> SDLPMPMRFRHLKKTSKEAVGVYRSPIHGRGLFCKRNIDAGEMVIEYAGIVIRSILTDKREKYYDSKGIGCYMFRIDDSEVVDATMHGNAARFINHSCEPNCYSRVINIDGQKHIVIFAMRKIYRGEELTYDYKFPIEDASNKLPCNCG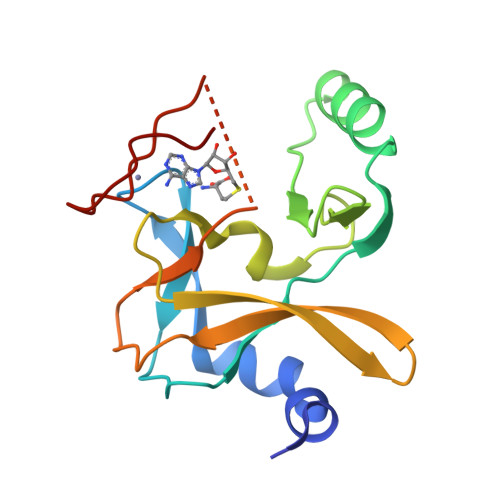AKKCRKFLN> MGSSHHHHHHSSGENLYFQGHMSNTSWRKSEVLAVPLQPTLQQEVILARMEQILASRALTDDERAQLLYERGVLYDSLGLRALARNDFSQALAIRPDMPEVFNYLGIYLTQAGNFDAAYEAFDSVLELDPTYNYAHLNRGIALYYGG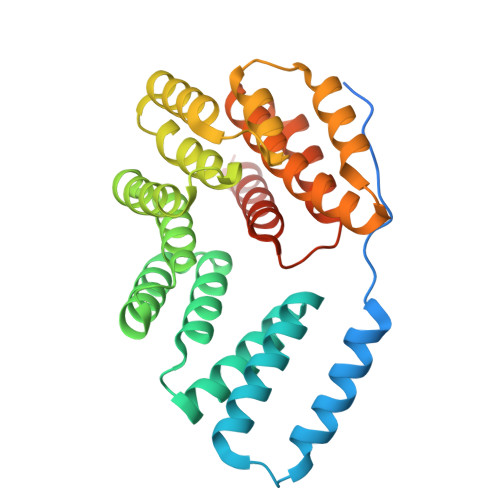RDKLAQDDLLAFYQDDPNDPFRSLWLYLAEQKLDEKQAKEVLKQHFEKSDKEQWGWNIVEFYLGNISEQTLMERLKADATDNTSLAEHLSETNFYLGKYYLSLGDLDSATALFKLAVANNVHNFVEHRYALLELSLLGQDQDDLAESDQQ> MNRYLGHGTRTSRENTNLSELHGILSLGLNVDHTIVRKKSIPLFEIGNSDQVCNWIIQIIEAGVDLQEVADSFLTMLCVNHAYQGDPNLFLESPAAHYLKGHGIHFEIQHRDNVDHITDLLGVGSRDKSLRKTLSALEFEPGGTTTAGMFLSFASLFLPKLVVGERACLEKVQRQIQIHAEQGLIQYPTQWQSVGHMMVVFRLIRVNFVLKFLLVHQGMHMMAGHDANDAIIANSISQTRFSGLLIVKTVLEHILQKTEAGVQLHPLARTSKVKGELLAFKSALEALASHREYAPFARLLNLSGVNNLEHGLYPQLSAIALGVATAHGSTLAGVNVSEQYQQLREAATEAEKQLQQHSEMRELETLGLDEQERKILATFHSRKNEINIQQTSSILAIRKERLRKLTEALTEEKNKNALDDEDESEEDDWSPENRGIRSNKGSTKEPSSYTASRTEEDRNNYNSKDDHLSGKEQMSTQQESGADDLDLFDLDDDGDTNSQDPNNRQKQSDTQQTQESSDRSDYSRRPAYDWPPGDRPHTTQATDEHTDLLNKDHRRNQVKPGRRGNDPRTLPLISFDDNEGEILDDKSDLPAPDTHSDPDTEESEEEHP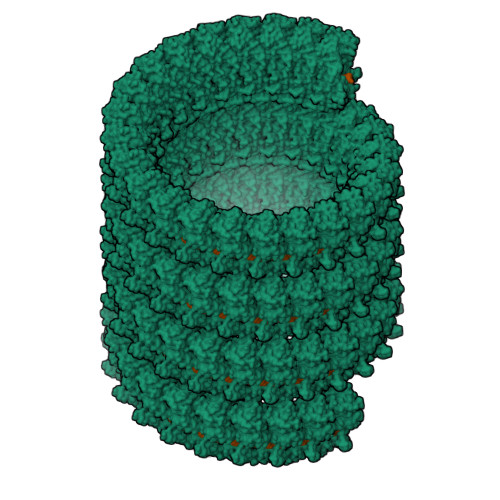DEELLPPAPKYSTKTSEQEPGDWKQPTSPLSTIPEEEGGHEANNDNSESDLIDQMYQHIFKTEGAYAAINYYYKTTGRPVTFTSNNNHDYTFPQDTEGLFPPWEGKENQKVAEILTNSLHETGQEWADMSAKERYLFLINN> GLPTHLYKNFTV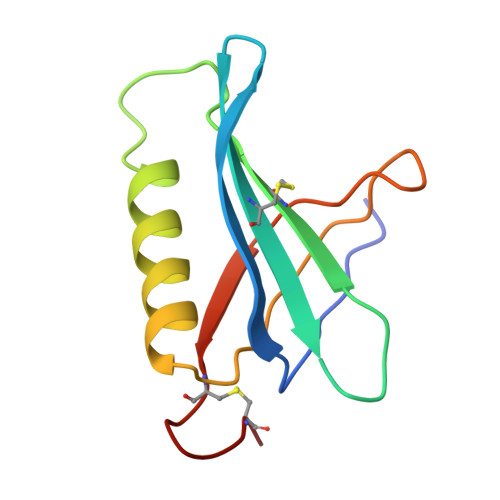QELALKLKGKNQEFCLTAFMSGRSLVRACLSDAGHEHDTWFDTMLGFAISAYALKSRIALTVEDSPYPGTPGDLLELQICPLNGYCE>GGRLFLHLKRSDNKPVPFGSIVTIEGQSSSSGIVGDNSGVYLTGLPKKSKILVKWGRDKNQSCSSNVVLPEKTDISGAYRLSTT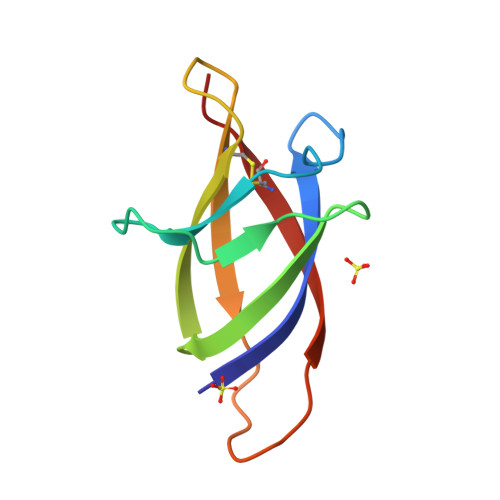CILNN[2x]>SNAIGGAVKLS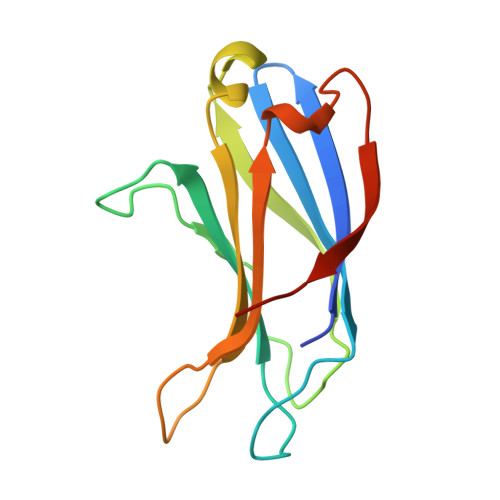ISYRNGTLFIMVMHIKDLVTEDGADPNPYVKTYLLPDNHKTSKRKTKISRKTRNPTFNEMLVYSGYSKETLRQRELQLSVLSAESLRGNFFLGGVTLPLKDFNLSKETVKWYQLTAATYL[3x]>RPQGATVSLWETVQKWREYRRQCQRSLTEDPPPATDLFCNRTFDEYACWPDGEPGSFVNVSCPW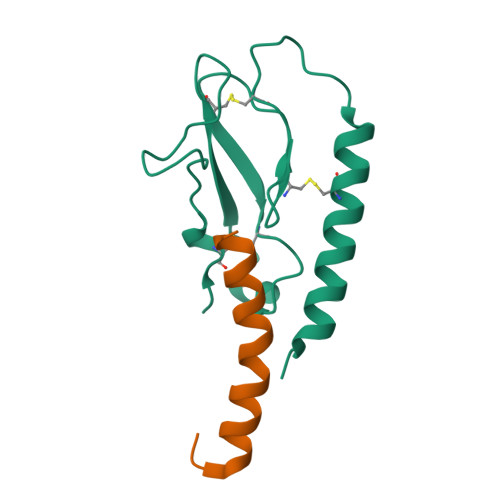YLPWASSVPQGHVYRFCTAEGLWLQKDNSSLPWRDLSECEESKRGERSSPEE[2x];>HCEGCFTSDVSSYLEGQAAKEFIAWLVKGRG[2x]>MGSSHHHHHHSSGLVPRGSHMKEAGQMQNLESARAGRSVSTQTGSMTGQIPRLSKVNLFTLLSLWMELFPAEAQRQKSQKNEEGKHGPLGDNEERTRVSTDKRQVKRTGLVVVKNMKIVGLHCSSEDLHAGQIALIKHGSRLKNCDLYFSRKPCSACLKMIVNAGVNRISYWPADPEISLLTEASSSEDAKLDAKAVERLKSNSRAHVCVLLQPLVCYMVQFVEETSYKCDFIQKITKTLPDANTDFYYECKQERIKEYEMLFLVSNEEMHKQILMTIGLENLCENPYFSNLRQNMKDLILLLATVASSVPNFKHFGFYRSNPEQINEIHNQSLPQEIARHCMVQARLLAYRTEDHKTGVGAVIWAEGKSRSCDGTGAMYFVGCGYNAFPVGSEYADFPHMDDKQKDREIRKFRYIIHAAQNALTFRCQEIKPEERSMIFVTKCPCDECVPLIKGAGIKQIYAGDVDVGKKKADISYMRFGELEGVSKFTWQLNPSGAYGLEQNEPERRENGVLRPVPQKEEQHQDKKLRLGIH[3x]

Vertebrates possess a second DCTD-like protein, CDADC1 (NYD-SP15). Unlike DCTD, CDADC1 contains two CMP/dCMP-like deaminase domains (IPR002125), connected by a long (>100 residues) linker within a single polypeptide chain, resulting in CDADC1 being approximately triple the length of DCTD (e.g. 514 residues in human CDADC1 versus 178 in human DCTD). The C-terminal deaminase domain (CTD) of CDADC1 contains a potentially active HAE motif, but its N-terminal domain (NTD) appears to be naturally inactivated due to the mutation of the proton shuttle glutamate (the HAG motif instead of HAE), suggesting noncatalytic function. In this work, we provide biochemical and structural evidence that human CDADC1 deaminates dCTP and CTP.

We collected datasets of the CDADC1 E400A variant alone, in the presence of dCTP (“good” substrate), and in the presence of 5mdCTP (“bad” substrate). All three datasets were analyzed imposing either C3 (trimer) or D3 (dimer of trimers, hexamer) symmetry. CDADC1 trimers are closed rings formed by three protomers assembled in a head-to-tail orientation. The majority of the contacts are formed between Nα2 and Nα3 from the NTD of one protomer and Cα2 and Cα3 of the CTD of the other. In addition, the structured portion of the loop 367–396 (369–375 and 391–396) near the CTD active site forms contacts with both Nα3 and Nα4 from the NTD. This results in the vast interface of ~1,100 Å2 between the two adjacent protomers, according to the PISA server. In our structures, the side chain of E400 is missing, because the residue was mutated to alanine to prevent catalysis. The trimer maps in the ligand binding region and the trimer conformation suggested a ligand-free state of the trimer, irrespective of whether or not dCTP or 5mdCTP was present in the sample. There is no evidence for ligand binding in the maps of the CTD active sites, and no significant structural changes seem to occur, suggesting that trimers do not bind dCTP or 5mdCTP.Bioluminescence light emission is produced through the catalysis of a small molecule substrate, most commonly D-luciferin (D-LH2), by a luciferase enzyme. We recently described the LH2 analogue infraluciferin (iLH2) which has a luciferase dependent red-shifted peak emission of up to 706 nm. In this work, we explored the possible structural interactions in the enzyme that may account for the near infrared emission of iLH2 and its application to dual-BLI in vivo. We described previously iLH2, which has a near-infrared emission and in contrast to other LH2 analogues maintains the 6’ hydroxyl benzothiazole group of LH2 that preserves the colour-shifts of mutant luciferases.

First, the X-ray crystal structure of FLuc in complex with a high-energy intermediate analogue, 5’-O-[(N-dehydroinfraluciferyl)-sulfamoyl] adenosine (iDLSA) was determined to provide insight into the FLuc-iLH2 light-emitting reaction. The structures show good alignment to each other, however there is evidence of a more open active site supported by a reduction in root-mean-squared (RMSD) score when aligned based on just the N-terminal domain of FLuc rather than the entire structure (RMSD = 0.688 and 0.783 respectively). All FLuc residues in close proximity (4 Å) to DLSA were also found to be within the same distance to iDLSA, with the exception of Arg437, >4 Å away from iDLSA. The altered position of the benzothiazole ring and the greater size of iDLSA may be the cause of a series of small active site changes that affect residues Glu311, Arg337, Asn338, Gly339, and Thr343 resulting in a total of six differences in H-bonding interactions. When specific residues implicated in the light emitting reaction were measured between the two structures differences ranged from 0.7 to 1.6 Å; with the biggest divergence being Lys529 (found in the C-terminal cap) which had a 2.4 Å difference in the nitrogen residue found in the side chain of the amino acid. Analysis of the x-ray crystal structure of FLuc in complex with the iLH2 analogue (iDLSA) revealed that the hydrogen-bonding network, thought to be critical in stabilising the phenolate ion of the emitter, is disrupted in the FLuc-iDLSA due to the accommodation of the larger iLH2 substrate. Evidence for the disruption of the network is the absence of a H-bond between Arg337 and Glu311 that is found in the DLSA structures of FLuc and L. cruciata Luc. In addition, the resulting increase in active site polarity due to the rotation of the C-terminal cap could also contribute to the red-shift in light emission. It must be noted that the crystal structure reported here has captured FLuc in the adenylation step of the reaction, therefore further computational modelling/crystal structure elucidation would be expected to provide further information on the light-emitting step of the reaction with iLH2.

>[2x]AKNIKKGPAPFYPLEDGTAGEQLHKAMKRYALVPGTIAFTDAHIEVNITYAEYFEMSVRLAEAMKRYGLNTNHRIVVCSENSLQFFMPVLGALFIGVAVAPANDIYNERELLNSMNISQPTVVFVSKKGLQKILNVQKKLPIIQKIIIMDSKTDYQGFQSMYTFVTSHLPPGFNEYDFVPESFDRDKTIALIMNSSGSTGLPKGVALPHRTACVRFSHARDPIFGNQIIPDTAILSVVPFHHGFGMFTTLGYLICGFRVVLMYRFEEELFLRSLQDYKIQSALLVPTLFSFFAKSTLIDKYDLSNLHEIASGGAPLSKEVGEAVAKRFHLPGIRQGYGLTETTSAILITPEGDDKPGAVGKVVPFFEAKVVDLDTGKTLGVNQRGELCVRGPMIMSGYVNNPEATNALIDKDGWLHSGDIAYWDEDEHFFIVDRLKSLIKYKGYQVAPAELESILLQHPNIFDAGVAGLPDDDAGELPAAVVVLEHGKTMTEKEIVDYVASQVTTAKKLRGGVVFVDEVPKGLTGKLDARKIREILIKAKKGG>[5x]MALTTTGTEQHDLFSGTFWQNPHPAYAALRAEDPVRKLALPDGPVWLLTRYADVREAFVDPRLSKDWRHRLPEDQRADMPATPTPMMILMDPPDHTRLRKL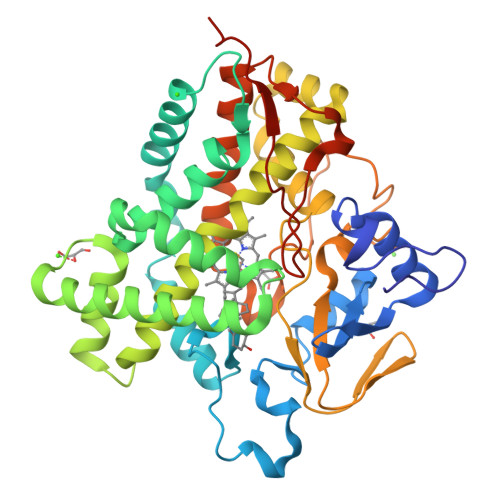VGRSFTVRRMNELEPRITEIADGLLAGLPTDGPVDLMREYAFQIPVQVICELLGLPAEDRDDFSAWSSVLVDDSPADDKNAAMGKLHGYLSDLLERKRTEPDDALLSSLLAVSDMDGDRLSQEELVAMAMLLLIAGHETTVNLIGNGVLALLTHPDQRKLLAEDPSLISSAVEEFLRFDSPVSQAPIRFTAEDVTYSGVTIPAGEMVMLGLAAANRDADWMPEPDRLDITRDASGGVFFGHGIHFCLGAQLARLEGRVAIGRLFADRPELALAVGLDELVYRRSTLVRGLSRMPVTMGPRSALEHHHHHH> MAQILPIRFQEHLQLQNLGINPANIGFSTLTMESDKFICIREKVGEQAQVVIIDMNDPSNPIRRPISADSAIMNPASKVIALKAGKTLQIFNIEMKSKMKAHTMTDDVTFWKWISLNTVALVTDNAVYHWSMEGESQPVKMFDRHSSLAGCQIINYRTDAKQKWLLLTGISAQQNRVVGAMQLYSVDRKVSQPIEGHAASFAQFKMEGNAEESTLFCFAVRGQAGGKLHIIEVGTPPTGNQPFP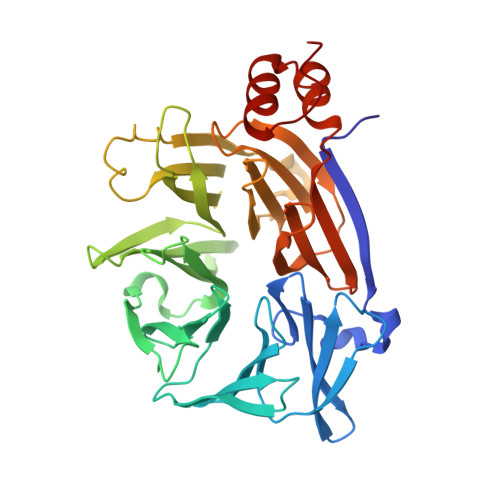KKAVDVFFPPEAQNDFPVAMQISEKHDVVFLITKYGYIHLYDLETGTCIYMNRISGETIFVTAPHEATAGIIGVNRKGQVLSVCVEEENIIPYITNVLQNPDLALRMAVRNNLAGAEELF> ADVHDKATRSKNMRAIATRDTAIEKRLASLLTGQGLAFRVQDASLPGRPDFVVDEYRCVIFTHGCFWHHHHCYLFKVPATRTEFWLEKIGKNVERDRRDISRLQELGWRVLIVWECALRGREKLTDEAL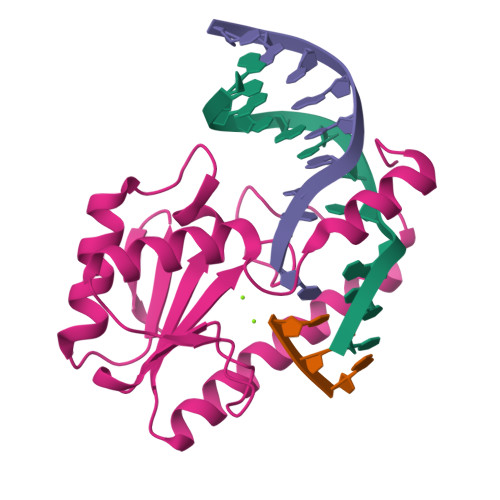TERLEEWICGEGASAQIDTQGIHLLA> QDRLDAPPPPAAPLPRWSGPIGVSWGLRAAAAGGAFPRGGRW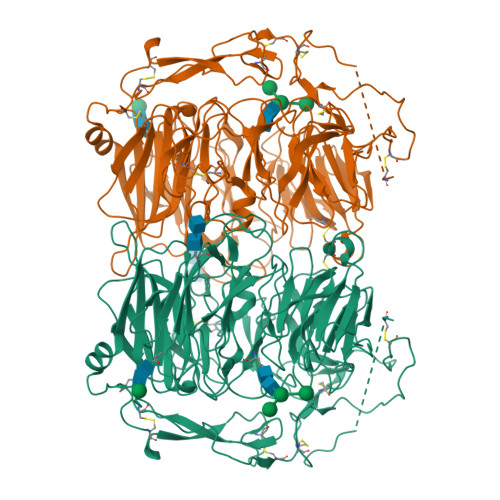GGSAPGEDEECGRVRDFVAKLANNTHQHVFDDLRGSVSLSWVGDSTGVILVLTTFHVPLVIMTFGQSKLYRSEDYGKNFKDITDLINNTFIRTEFGMAIGPENSGKVVLTAEVSGGSRGGRIFRSSDFAKNFVQTDLPFHPLTQMMYSPQNSDYLLALSTENGLWVSKNFGGKWEEIHKAVCLAKWGSDNTIFFTTYANGSCKADLGALELWRTSDLGKSFKTIGVKIYSFGLGGRFLFASVMADKDTTRRIHVSTDQGDTWSMAQLPSVGQEQFYSILAANDDMVFMHVDEPGDTGFGTIFTSDDRGIVYSKSLDRHLYTTTGGETDFTNVTSLRGVYITSVLSEDNSIQTMITFDQGGRWTHLRKPENSECDATAKNKNECSLHIHASYSISQKLNVPMAPLSEPNAVGIVIAHGSVGDAISVMVPDVYISDDGGYSWTKMLEGPHYYTILDSGGIIVAIEHSSRPINVIKFSTDEGQCWQTYTFTRDPIYFTGLASEPGARSMNISIWGFTESFLTSQWVSYTIDFKDILERNCEEKDYTIWLAHSTDPEDYEDGCILGYKEQFLRLRKSSMCQNGRDYVVTKQPSICLCSLEDFLCDFGYYRPENDSKCVEQPELKGHDLEFCLYGREEHLTTNGYRKIPGDKCQGGVNPVREVKDLKKKCTSNFLSPEKQNSKSNS>MIKRLFSKSKPATIEQTPTPEKTPYEILGGEAGALAIANRFYDIMATDEYAKPLYDMHPLPLDRIRQVFFEFLSGWLGGP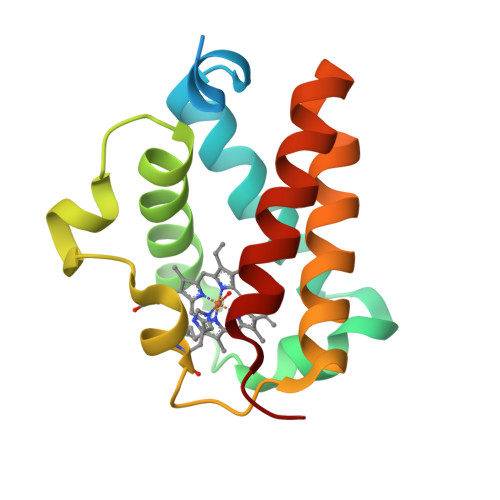DLFVAKHGHPMLRKRHMPFTIDQDLRDQWMYCMNKTLDLEVDNPLLREGLKQSFGQLASHMINQH[2x]> MDD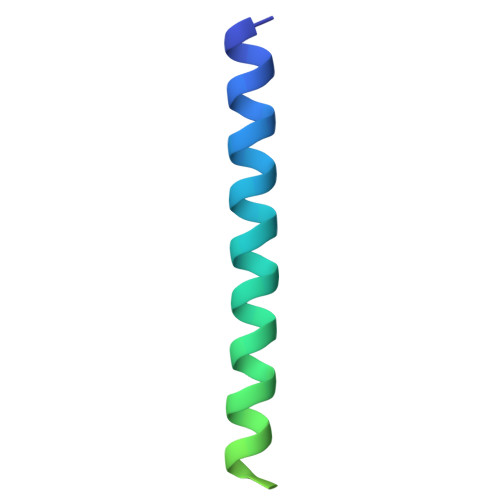LAQTKAIKDQLQKYIRELEQANDDLERAKRATIMSLEDFEQRLNQAIERNAFLESELDEKENLLESVQR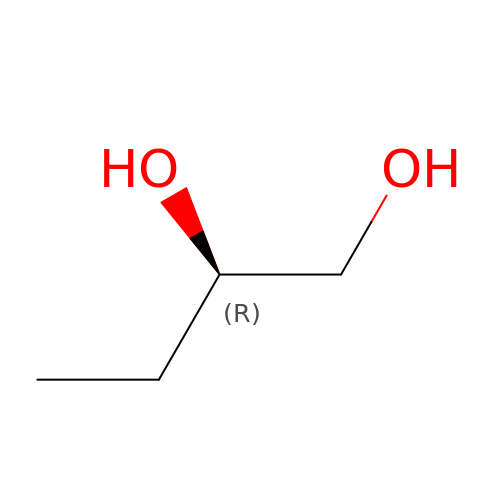(2~{R})-butane-1,2-diol | C4 H10 O2 | BMRWNKZVCUKKSR-SCSAIBSYSA-N> DPGCLPDWSSYKGHCYKVFKKVGTWEDAEKFCVENSGHLASIDSKEEADFVTKLASQTLTKFVYDAWIGLRDESKTQQCSPQWTDGSSVVYENV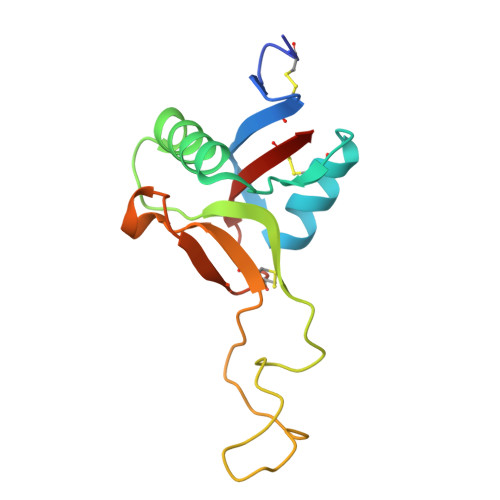DEPTKCFGLDVHTEYRTWTDLPCGEKNPFICKSRLPH>QNVSLQPPPQQLIVQNKTIDLPAVYQLNGGEEANPHAVKVLKELLSGKQSSKKGMLISIGEKGDKSVRKYSRQIPDHKEGYYLSVNEKEIVLAGNDERGTYYALQTFAQLLKDGKLPEVEIKDYPSVRYRGVVEGFYGTPWSHQARLSQLKFYGKNKMNTYIYGPKDDPYHSAPNWRLPYPDKEAAQLQELVAVANENEVDFVWAIHPGQDIKWNKEDRDLLLAKFEKMYQLGVRSFAVFFDDISGEGTNPQKQAELLNYIDEKFAQVKPDINQLVMCPTEYNKSWSNPNGNYLTTLGDKLNPSIQIMWTGDRVISDITRDGISWINERIKRPAYIWWNFPVSDYVRDHLLLGPVYGNDTTIAKEMSGFVTNPMEHAESSKIAIYSVASYAWNPAKYDTWQTWKDAIRTILPSAAEELECFAMHNSDLGPNGHGYRREESMDIQPAAERFLKAFKEGKNYDKADFETLQYTFERMKESADILLMNTENKPLIVEITPWVHQFKLTAEMGEEVLKMVEGRNESYFLRKYNHVKALQQQMFYIDQTSNQNPYQPGVKTATRVIKPLIDRTFATVVKFFNQKFNAHLDATTDYMPHKMISNVEQIKNLPLQVKANRVLISPANEVVKWAAGNSVEIELDAIYPGENIQINFGKDAPCTWGRLEISTDGKE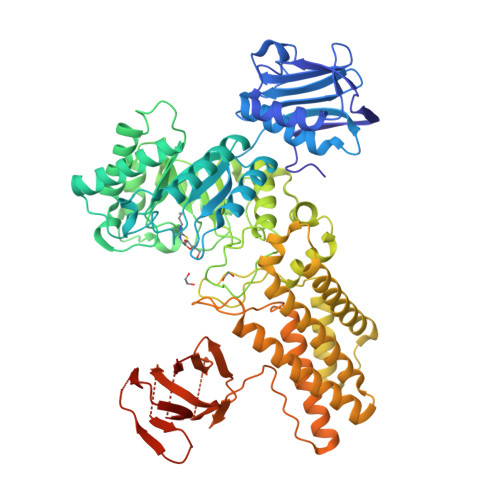WKTVDLKQKESRLSAGLQKAPVKFVRFTNVSDEEQQVYLRQFVLTIEKK[2x]> FTDYKVADITLAAWGRRELIIAESEMPALMGLRRKYAGQQPLKGAKILGCIHMTIQTGVLI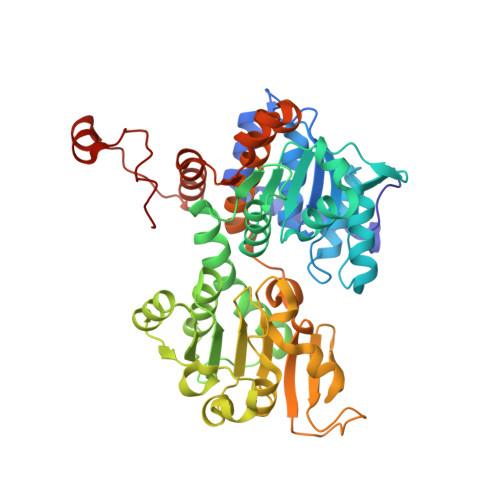ETLVALGAEVRWSSCNIFSTQDQAAAAIAAAGIPVFAWKGETEEEYEWCIEQTILKDGQPWDANMVLDDGGDLTEILHKKYPQMLERIHGITEETTTGVHRLLDMLKNGTLKVPAINVNDSVTKSKNDNKYGCRHSLNDAIKRGTDHLLSGKQALVIGYGDVGKGSSQSLRQEGMIVKVAEVDPICAMQACMDGFEVVSPYKNGINDGTEASIDAALLGKIDLIVTTTGNVNVCDANMLKALKKRAVVCNIGHFDNEIDTAFMRKNWAWEEVKPQVHKIHRTGKDGFDAHNDDYLILLAEGRLVNLGNATGHPSRIMDGSFANQVLAQIHLFEQKYADLPAAEKAKRLSVEVLPKKLDEEVALEMVKGFGGVVTQLTPKQAEYIGVSVEGPFKPDTYRY> MATAGNPWGWFLGYLILGVAGSLVSGSCSQIINGEDCSPHSQPWQAALVMENELFCSGVLVHPQWVLSAAHCFQNSYTIGLGLHSLEADQEPGSQMVEASLSVRHPEYNRPLLANDLMLIKLDESVSESDTIRSISIASQCPTAGNSCLVSGWGLLANGRMPTVLQCVNVSVVSEEVCSKLYDPLYHPSMFCAGGGHDQKDSCNGDSGGPLICNGYLQGLV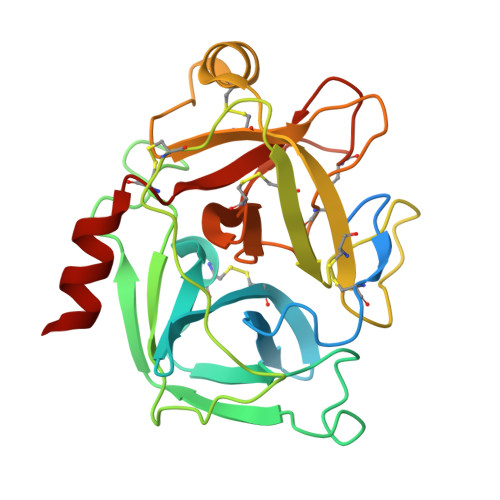SFGKAPCGQVGVPGVYTNLCKFTEWIEKTVQAS>[2x]GSSSGGSGHTPTTQATHADDHDLTTHNGTEEHDDGHDDGHDDLHAHAPKVIVFISGSCLFGAISRSLFKKLPIPYTVVLLILGAILGVVASNVPLVEEHTRDVAHMDPHVLLQIFLPVLIFESAFAMDVHTFMRSFSQVCILALFGLVVASVLTAVLAMNLFNYNWNFSEAMMFGAIMSATDPVAVVALLKDLGASKQLGTIIEGESLLNDGCAIVIFNVFMKMVFFPQLTSTVGQNVLYFLQVAVAGPLWGYAVAKVTVFFLSHIFNDALVEITITLAATYLTYYIGDIWLEVSGVLAVVVLGLIVNAEKTSISPEVEVFLHRFWEMLAYLANTLIFMMVGVVVTQKALVAVDKMDWFYLIILYLAITIIRGMVISLFSPILSRIGYGLTWRNAVIMTWGGLRGAVGLALALVVENLAGNDVIGSKFLFHTAGIVVLTLVINATTIQTLLRILGMSDISIPKRLAMAGAVRRIHEGQNRTLNMLKSDRFLADADWDIATAACEISDPYSALSDDENAPADELTLGERKSVCPGCKAMVPNEPSPREFADMMEEARLRMLKAEKISYWKQFEHGMLAREALRLLVQHAEVAADEKDQFILVDDLKKSWQIKGIYPWLKRKLEDLISEKKIAAIPMPKYKLGKLMYKICHHMAFEVTINIAIVLNIVPIIMEFVVQDKMASVSTMAAPGSTVSSEPSSLQKIEDALRISNYVFFVIYAIEAIVKILGLGRHYIVSHWNKFDAFILVVALVDIIIAETLLKGSITINLSSIKVVKLFRLLRGLRMLRLTKALIPKLILVVNGKINNQLSLGYDVGKGYIIGEEEVGKIIDRMVDNKKILRELKHISETGRLQVVKELGLLQREHPGIAVSVKTRQAIRTILNHSRETIH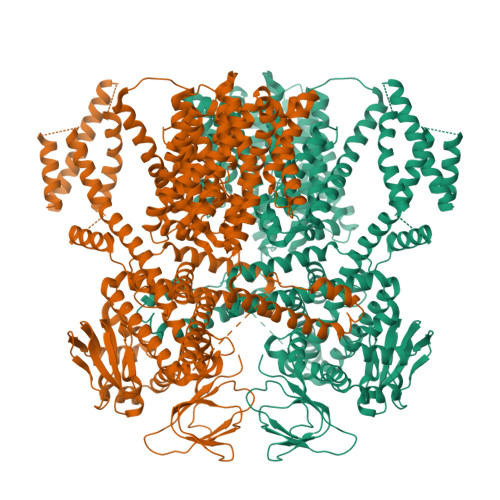ELQGAGLLDEMEAHKLELTVEIKMKRLMNAPSSIPPPPPENLLKNVSWLAGDMKLIDFIKARASLLHFDYGEVIVREGDESDGLFLIVSGLVKLYGKSAFLDHDNPPVTAGSEENEVFEDYLTVGNVIGEMGVLTKKPRNATVTCETTVQVYFITAEDMNIAIDTFTLYPSLEYRLWRVVAIRIATPLIMEQMAFQGWTQEKVKLHLERGYLVDLAESHFQFNIDATLEDVILINGTAYNAHTREEIRSPCLISRTVHKLTFQYTATEEPRLFVVRNAEYNGPILDGRLDVDSKRSLISITEISSNMCLKHAAELRQKNSKVMLSRKSSGAAAKEEEDCIPNTSDVEQAAGVSPSVPTKTTPKPKSFLPSLGLSMSKERVNGEAVEESPVKTKQGEETPETEEGAAPRVNVASNSLEVLFQ>[2x]IVPTRELENVFLGRCKDYEITRYLDILPRVRSDCSALWKDFFKAFSFKNPCDLDLGSYKDFFTSAQQQLPKNKVMFWSGVYDEAHDYANTGRKYITLEDTLPGYMLNSLVWCGQRANPGFNEKVCPDFKTCPVQARESFWGMASSSYAHSAEGEVTYMVDGSNPKVPAYRPDSFFGKYALPNLTNKVTRVKVIVLHRLGEKIIEKCGAGSLLDLEKLVKAKHFAFDCVENPRAVLFLLCS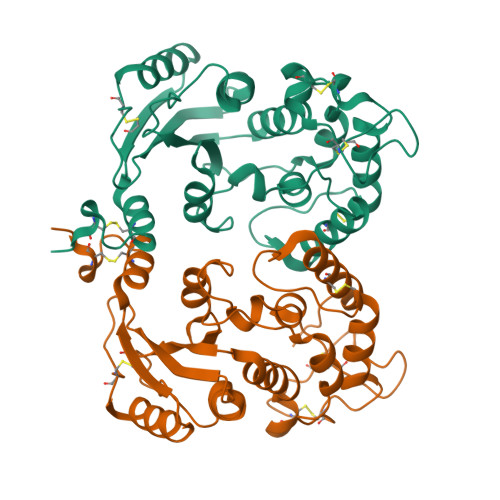DNPNARECRLAKRFYRIA> MAAQLALNSEASLWGPYREIWQTVLSALIKRQPEAVHSLDIVLKKYKPDFISLFKNPPKSAQQHERVQKASTEGIPIKGTQRTRILEEQLIKEAFILSDLYNIGEIAAVELLLIGEQQQPTFHGLTRGLVAILLYWDGKSCMAESLLHLIQARKGKTFTLDHSPEVVSMVTRFTDDLMEQGLTNKILTLISQIDVNNEFDKLKKERGLGNKKHRKEVSDLIKECQQSLAHSLYSWSCQTPLNREDTLLLIGYLEKVTVEGDGSLDKVNLTLLMSLLYCLDVGFLEQGTDDREELMKQASMFMDRQYIAAIHNRLQNTQPWKSPGMQATVRLAWALALRGISQFSEVLEFSEADEPMAEIAIGGNVFLFLTEAVVGSESFCTDEFFIRRIHKLVTDFPTLMPMKVKQLRNRAEEDARLIQMSMQMGNEPPASLRRDLEHLLLLIGELYRKDPFHLELALEYWCPTEPLQSTSLMGSFLGVAHQRPPQRQVLLSKFVRQMSDLLPATLYLPYLKMLRGLASGPQCAHYCFSLLKANGGSSAENLQAAGGSPVSWDHFFHSLMLYHEHLRRDLPNTDNIHQRHPPLRGITQRELDGLIACLQLTCTIIDWSESARLALCEHAQWMPVVVILGLLQCSIPPLLKAELLKTLAAFGKSPEIAASLWQSLEYTQILQTVRATGLRQGVGIEVELNEIESRCEEYPLTRAFCQLISTLVESSFPTNLGAGLRAPGFEPYLQFLRDTVFLRYRTRAYRRAAEKWEVAEAVLDVFYKLLKDYEPQPEDFVDQYVELQGEERVAFKPPGFSLMHHLLNESPMLELCLSLMEEGVTQLDTYAPFPGKKHLEKAVAYCFMLLNLTLQKENRFMDLLRESHLSMIVTPLEQLLQGINPRSKKADNVVNIARYLCHGNSNAELAFESAKILCSISCNSKIQEKIVGDFTQDQNVSQKLMVGFVSCLDSEEAEELLDSEKEAEDQVKQTNIRYMTKIHILNLLITSLEMKAPNLAMFLLGYELKKPVSTTNLQDSGVLGCPRTCLHSILDILRKGTDVRAGPVAVWDTPHLAELCYQVIYQLCACADTSGPTMRYLRTSQDFLFSQLQHLPFSVEESEISAMNQMSWLMKTATIELRITSLNRQRSHTQRLLHLLLDDMPTRPYSAD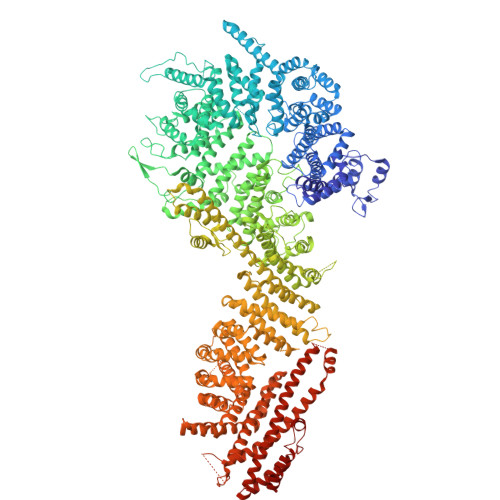GEGGMEDESRSLSGFLHFDTTSKVRRKILRILDSIQFSNEIPEPLQLDFFDRSQIEQVIANCEHKNRRGQTVCNVKLLHRVLVAEVNALQGMAAIGQRPLLMEEINTILQYVVERNKLLQCLHAKRHALESWRQLVEIILTACPQDLIPTEHRQLIIRDLLQDLHVKILDDDAAQELMPIVAGAVFTLTAHLSQSVRTELKQPMTASGLGQSQYVQMLDGSFAAPPGTENISAGFASIGDSSLHMILRNLLEFILKTGGGFQRVRAHLYGSLLYYLQIAQRPDEPDTLESAHKSMWERLTAPEDVFSKLQRDNLSIFESYGTALMEVVCRDACDGHDIGRMLALALLDRIVSVDRQQQWLLYLSNSGYLKVLVDSLAEDDVVLRNLLTPQPPLLKALYIYESKMAFLTRVAKSSQGAIELLRSGVIVRLAQCQVYDMRPETDPHGVFGMRETPVFIPAPVERYRQILLPALQICQLILTSSTAQHLQAAGQVLQFLVAHSDTIQAILRSQEGSLGSLQELALLTGIISKAALPGVLNELDIGLNDGSMMELQGHIGRFQRQCLALLNRFGGSDRLRQLSLQDDSSRLDGVSKKDDMELAMQQICSNVMEYCQALMIQNSPSFQQTVCLFTPSLKESASRDGTRQDSQVSILPSWRLPSLGVVIHLLKQSANNFFTYYDIHRQSVGKLQNVEQLPPDEIKELCQSEMPVGADKISTTQKYGLARRRLVKLINSRAKLLSLCSYIIETCLYILWRHLEYYLLHCTTSDSQDPVFSNMTFGNRRFQDTFNTDPNMDPRNLRQNKVSQQDVDTLLREGANSFGESLQKRLLDIESLYCKVRSRHSFIQALVRRIRGLLRVSRV> K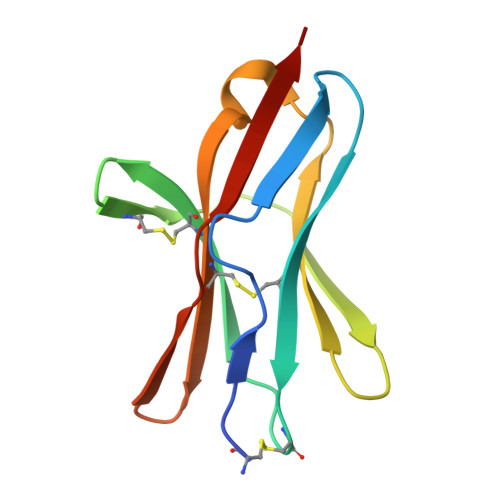ESCDVQLYIKRQSEHSILAGDPFELECPVKYCANRPHVTWCKLNGTTCVKLEDRQTSWKEEKNISFFILHFEPVLPNDNGSYRCSANFQSNLIESHSTTLYVTDVK> PNSMKNIESLFDYSAGQFEFIDHLLTMGVGVHFAALIFFLVVSQFVAPKYRIATALSCIVMVSAGLILNSQAVMWTDAYAYVDGSYQLQDLTFSNGYRYVNWMADIPCLLLQLLIVLNLKGKE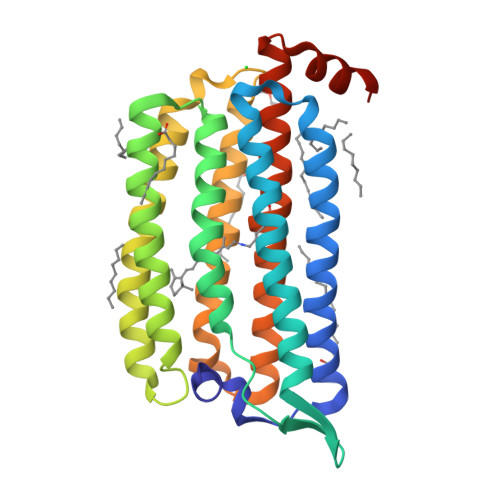LFSTATWLILAAWGMIITGYVGQLYEVDDIAQLMIWGAVSTAFFVVMNWIVGTKIFKNRATMLGGTDSTITKVFWLMMFAWTLYPIAYLVPAFMNNADGVVLRQLLFTIADISSKVIYGLMITYIAIQQSAAAGYVPAQQALGRIGMDSKAA>PELPEVETSRRGIEPHLVGATILHAVVRNGRLRWPVSEEIYRLSDQPVLSVQRRAKYLLLELPEGWIIIHLGMSGSLRILPEELPPEKHDHV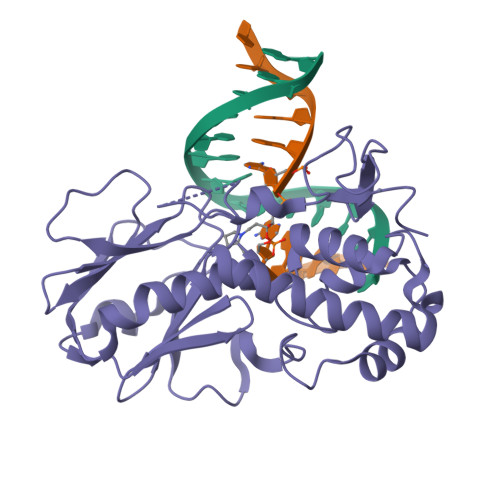DLVMSNGKVLRYTDPRRFGAWLWTKELEGHNVLTHLGPEPLSDDFNGEYLHQKCAKKKTAIKPWLMDNKLVVGVGNIYASESLFAAGIHPDRLASSLSLAECELLARVIKAVLLRSIEQGGTTLKDFLQSDGKPGYFAQELQVYGRKGEPCRVCGTPIVATKHAQRATFYCRQCQK[4x]>SNAMAEIKITPEELERIAGNFKNAAGEAQSQINRL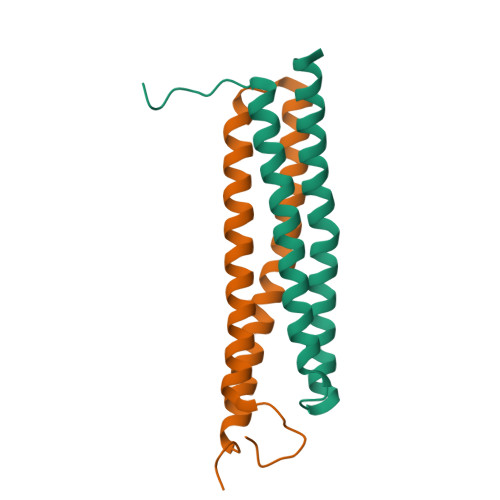EGDINSLEGQWAGATQAKFRGEFIQSKQAMQQYIPILEGISTDLKRIADKFRNTDNAY[4x]>[2x]SKKVDDLKNEFKETDKSARLTTDYGVKQTTADDWLRIVSDDKIGPSLLEDPFARERIMRFDHERIPERVVHARGSGAFGKFKVYESASDLTMAPVLTDTSRETPVFVRFSTVLGSRGSADTVRDVRGFAVKFYTEEGNWDLVGNNIPVFFIQDAIKFPDVIHAGKPEPHNEVPQAQSAHNNFWDFQFNHTEATHMFTWAMSDRAIPRSLRMMQGFGVNTYTLINAQGKRHFVKFHWTPELGVHSLVWDEALKLAGQDPDFHRKDLWEAIENGAYPKWKFGIQAIAEEDEHKFDFDILDATKIWPEDLVPVRYIGEMELNRNPDEFFPQTEQIAFCTSHVVN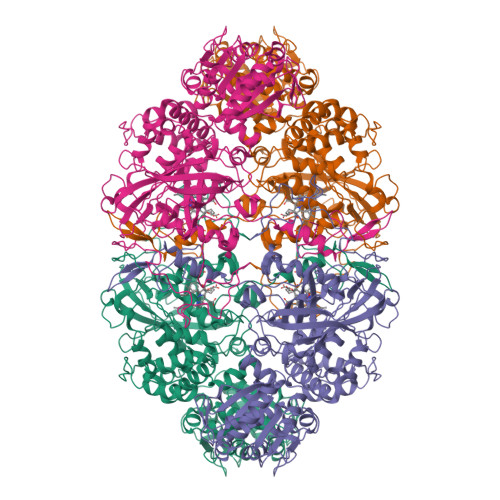GIGFSDDPLLQGRNFSYFDTQISRLGVNFQELPINRPVCPVMNFNRDGAMRHTISRGTVNYYPNRFDACPPASLKEGGYLEYAQKVAGIKARARSAKFKEHFSQAQLFYNSMSPIEKQHMINAFGFELDHCEDPVVYGRMVQRLADIDLGLAQTIAEMVGGEAPTTTNHPNHGRKTINLSQTEFPPATPTIKSRRVAIIIADGYDNVAYDAAYAAISANQAIPLVIGPRRSKVTAANGSTVQPHHHLEGFRSTMVDAIFIPGGAKAAETLSKNGRALHWIREAFGHLKAIGATGEAVDLVAKAIALPQVTVSSEAEVHESYGVVTLKKVKPESFTDAVKIAKGAAGFLGEFFYAIAQHRNWDRELDGLHSMIAY> STVYNINLGIGWASSGVEYAQAYRAQILRRIQQPAKFIFMDMILADNIQHLTENIGFLDEEIIWLYNYFTDIKIAPTTVTLDQVLAQVAGQPERSEKEGKIVRYFYPQDDQFITCYLRQEDQDFVEHVEYVSRGRLIRKDYFSYVRYASEYFAPHNDAATLYQRRFYHEDGSVAYDM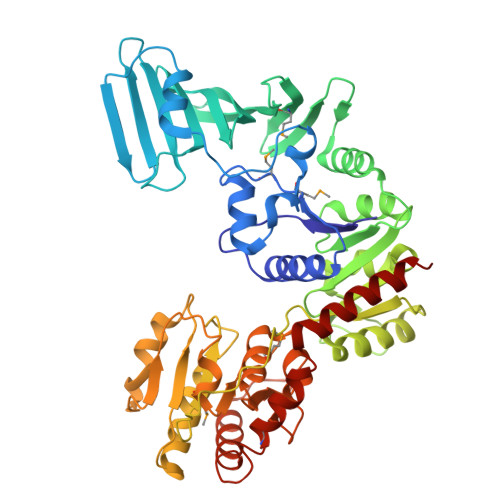LIEDGQEKLYRFPDRIFYSKAELVRYFLQCLQLQADDVVILDRETGIGQVVFEESQKAKLGVVVHAEHFSENASSDDYILWNNFYDYQFTNADKVDFFIVATEAQKRILEQQFQHYSDKQPQIATIPVGSLDQLTYPKEPRKPYSMITASRLATEKHIDWLVAATVQAHAQLPELTLDIYGKGSEEDKLRRRIEEAGAQDYIRLKGHADLSQIYAGYELYLTASTSEGFGLTLMEAVGSGLPLIGFDVRYGNQTFIDDGKNGYLLPVSSNHVEDQIIAAFVEKIIALFSQGRQQEMSQHSYQVAENYLTSRVEAAWTQLLKEVRDD> CGGAUUUAGCUCAGUUGGGAGAGCGC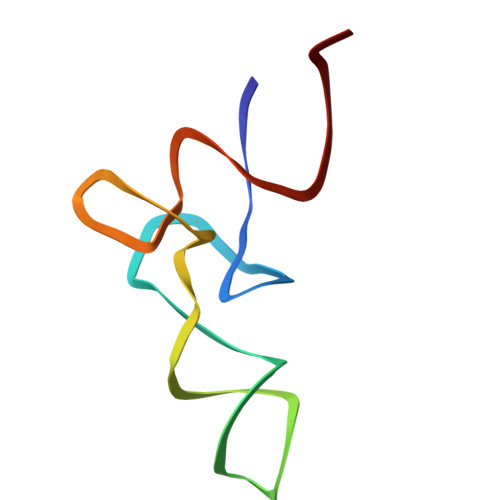CAGACUGAAGAUCUGGAGGUCCUGUGUUCGAUCCACAGAAUUCGCACCA>[14x]MNLIPTVIEQSSRGERAYDIYSRLLKDRIIMLSGQVTDDLANSIIAQLLFLDAQDSEKDIYLYINSPGGSVTAGMAIYDTMNFVKADVQTIVMGMAA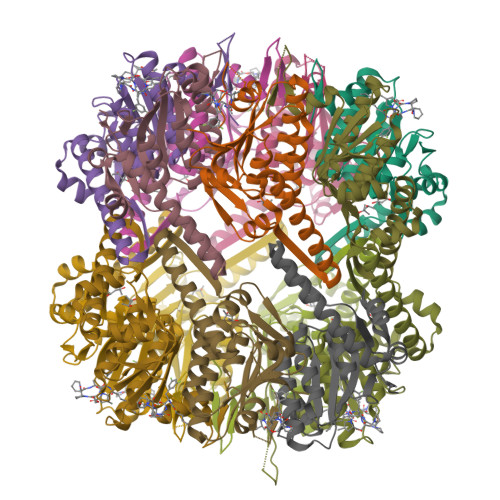SMGSFLLTAGTKGKRFALPNAEIMIHQPLGGAQGQATEIEIAARHILQTRERLNKILAERTGQPLEVIEKDTDRDNYMTAEQAKAYGLIDEVMENSSSLKIEGRGLEHHHHHH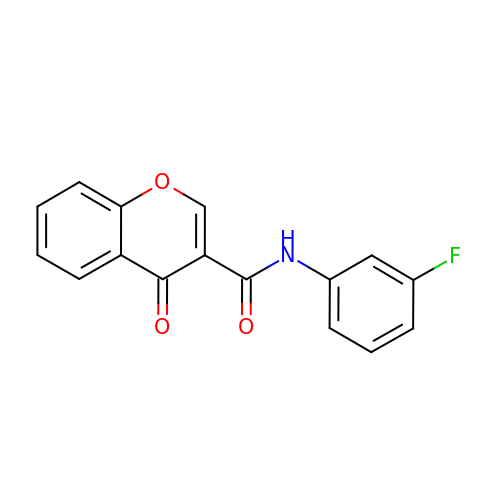~{N}-(3-fluorophenyl)-4-oxidanylidene-chromene-3-carboxamide | C16 H10 F N O3 | OUROIBLACYVZRJ-UHFFFAOYSA-N>MSQPRTPEQALDTPGDCPPGRRDEDAGEGIQCSQRMLSFSDALLSIIATVMILPVTHTEISPEQQFDRSVQRLLATRIAVYLMTFLIVTVAWAAHTRLFQVVGKTDDTLALLNLACMMTITFLPYTFSLMVTFPDVPLGIFLFCVCVIAIGVVQALIVGYAFHFPHLLSPQIQRSAHRALYRRHVLGIVLQGPALCFAAAIFSLFFVPLSYLLMVTVILLPYVSKVTGWCRDRLLGHREPSAHPVEVFSFDLHEPLSKERVEAFSDGVYAIVATLLILDICEDNVPDPKDVKERFSGSLVAALSATGPRFLAYFGSFATVGLLWFAHHSLFLHVRKATRAMGLLNTLSLAFVGGLPLAYQQTSAFARQPRDELERVRVSCTIIFLASIFQLAMWTTALLHQAETLQPSVWFGGREHVLMFAKLALYPCASLLAFASTCLLSRFSVGIFHLMQIAVPCAFLLLRLLVGLALATLRVLRGLARPEHPPPAPTGQDDPQSQLLPAPC[2x];>[2x]MAAPGSARRPLLLLLLLLLLGLMHCASAAMFMVKNGNGTACIMANFSAAFSVNYDTKSGPKNMTFDLPSDATVVLNRSSCGKENTSDPSLVIAFGRGHTLTLNFTRNATRYSVQLMSFVYNLSDTHLFPNASSKEIKTVESITDIRADIDKKYRCVSGTQVHMNNVTVTLHDATIQAYLSNSSFSRGETRCEQDRPSPTTAPPAPPSPSPSPVPKSPSVDKYNVSGTNGTCLLASMGLQLNLTYERKDNTTVTRLL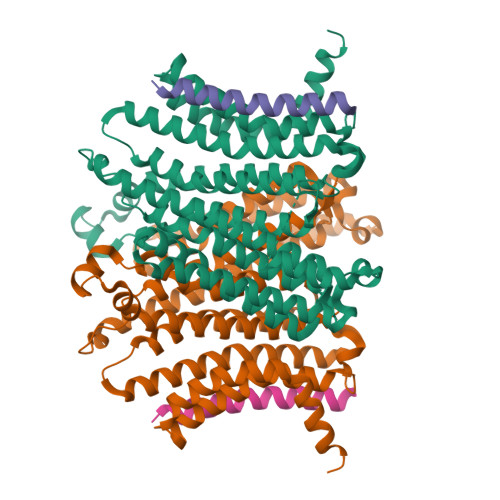NINPNKTSASGSCGAHLVTLELHSEGTTVLLFQFGMNASSSRFFLQGIQLNTILPDARDPAFKAANGSLRALQATVGNSYKCNAEEHVRVTKAFSVNIFKVWVQAFKVEGGQFGSVEECLLDENSMLIPIAVGGALAGLVLIVLIAYLVGRKRSHAGYQTI>GSQEKAVVLDEQAIRRALTRIAHEMIERNKGMNNCILVGIKTRGIYLAKRLAERIEQIEGNKVTVGELDITLYRDDLTKTSNKEPLVKGADIPVDITDQKVILVDDVLYTGRTVRAAMDALVDVGRPSSIQLAVLVDRGHRELPIRADYIGKNIPTSKSEKVMVQLSEVDG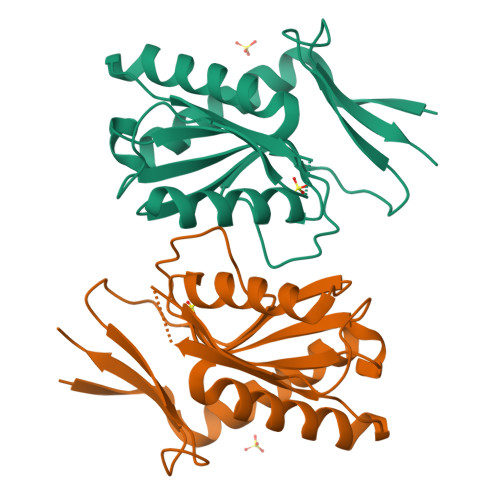QDLVAIYEK[2x]>MGLSLPKEKGLILCLWSKFCRWFQRRESWAQSRDEQNLLQQKRIWESPLLLAAKDNDVQALNKLLKYEDCKVHQRGAMGETALHIAALYDNLEAAMVLMEAAPELVFEPMTSELYEGQTALHIAVVNQNMNLVRALLARRASVSARATGTAFRRSPCNLIYFGEHPLSFAACVNSEEIVRLLIEHGADIRAQDSLGNTVLHILILQPNKTFACQMYNLLLSYDRHGDHLQPLDLVPNHQGLTPFKLAGVEGNTVMFQHLMQKRKHTQWTYGPLTSTLYDLTEIDSSGDEQSLLELIITTKKREARQILDQTPVKELVSLKWKRYGRPYFCMLGAIYLLYIICFTMCCIYRPLKPRTNNRTSPRDNTLLQQKLLQEAYMTPKDDIRLVGELVTVIGAIIILLVEVPDIFRMGVTRFFGQTILGGPFHVLIITYAFMVLVTMVMRLISASGEVVPMSFALVLGWCNVMYFARGFQMLGPFTIMIQKMIFGDLMRFCWLMAVVILGFASAFYIIFQTEDPEELGHFYDYPMALFSTFELFLTIIDGPANYNVDLPFMYSITYAAFAIIATLLMLNLLIAMMGDTHWRVAHERDELWRAQIVATTVMLERKLPRCLWPRSGICGREYGLGDRWFLRVEDRQDLNRQRIQRYAQAFHTRGSEDLDKDSVEKLVPRGSAAAWSHPQFEK[4x]

TRPV6 is a calcium-selective ion channel implicated in epithelial Ca2+ uptake. TRPV6 is a representative of the vanilloid subfamily of transient receptor potential (TRP) channels that is considered the principal epithelial calcium channel for Ca2+ absorption in intestines and many other organs. The channel is assembled of four subunits and contains two main components: a TMD with a central ion channel pore and an intracellular skirt that is mostly built of ankyrin repeat domains connected to each other by three-stranded β-sheets, N-terminal helices, and C-terminal hooks. The TMD is composed of six transmembrane helices S1–S6 and a re-entrant pore loop (P-loop) between S5 and S6.

In contrast, RR inhibits TRPV6 by binding in the middle of the ion channel’s selectivity filter and plugging its pore like a bottle cork. Compared with the open-state structure, the structure solved in the presence of RR showed a distinct non-protein density in the middle of the ion channel pore that perfectly matched the shape of RR. High-resolution reconstruction of TRPV6RR allows precise placement of the inhibitor inside the ion channel pore. On the extracellular side, the RR-binding site is flanked by aspartates D542 with a spherical density on the top that might represent a calcium ion typically bound at D542 in the absence of RR. The inhibitor occupies the entire selectivity filter of TRPV6, which is lined by carboxyl groups of D542, backbone carbonyl oxygens of I541, I540, and T539 as well as the hydroxyl group of T539, and spans the upper half of the pore’s central cavity. The surface of the selectivity filter is highly electronegative, creating a favorable environment for the positively charged RR that carries a 6+ total charge. In contrast, the pores in TRPV6RR and TRPV6Eco were apparently closed due to a hydrophobic seal imposed by the gate residues L574 and M578. Correspondingly, S6 in TRPV6RR and TRPV6Eco was entirely α-helical, typical for the closed conformation of TRPV6. We hypothesize that the positive charge of RR creates an electric field inside the pore’s central cavity that interacts with the electric dipole of the S6 helix. This interaction causes repulsion of the lower portion of S6 away from RR, which results in partial S6 rotation and helps S6 to become completely α-helical, with side chains of L574 and M578 sealing the pore.>[4x]MLRAAARFGPRLGRRLLSAAATQAVPAPNQQPEVFCNQIFINNEWHDAVSRKTFPTVNPSTGEVICQVAEGDKEDVDKAVKAARAAFQLGSPWRRMDASHRGRLLNRLADLIERDRTYLAALETLDNGKPYVISYLVDLDMVLKCLRYYAGWADKYHGKTIPIDGDFFSYTRHEPVGVCGQIIPWNFPLLMQAWKLGPALATGNVVVMKVAEQTPLTALYVANLIKEAGFPPGVVNIVPGFGPTAGAAIASHEDVDKVAFTGSTEIGRVIQVAAGSS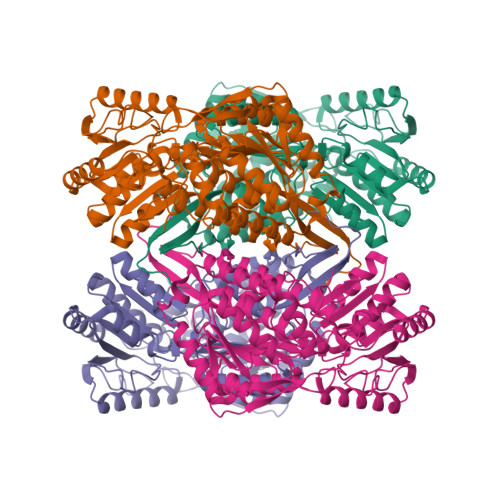NLKRVTLELGGKSPNIIMSDADMDWAVEQAHFALFFNQGQCCCAGSRTFVQEDIYDEFVERSVARAKSRVVGNPFDSKTEQGPQVDETQFKKILGYINTGKQEGAKLLCGGGIAADRGYFIQPTVFGDVQDGMTIAKEEIFGPVMQILKFKTIEEVVGRANNSTYGLAAAVFTKDLDKANYLSQALQAGTVWVNCYDVFGAQSPFGGYKMSGSGRELGEYGLQAYTEVKTVTVKVPQKNS4-{[3-chloro-4-(alpha-D-mannopyranosyloxy)phenyl]carbamoyl}benzoic 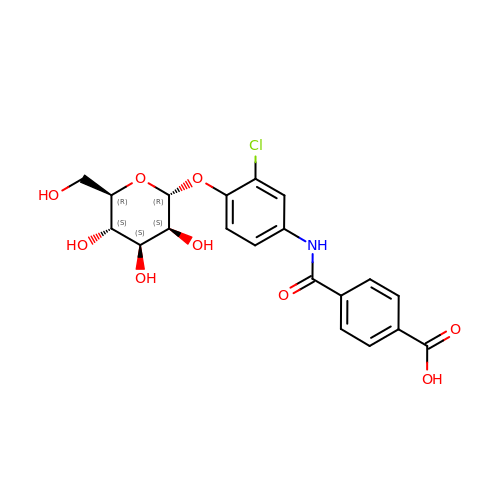acid | C20 H20 Cl N O9 | HIKPKPMJGGGESU-BAPGRXHISA-N> SHMKFTVEREHLLKPLQQVSGPLGGRPTLP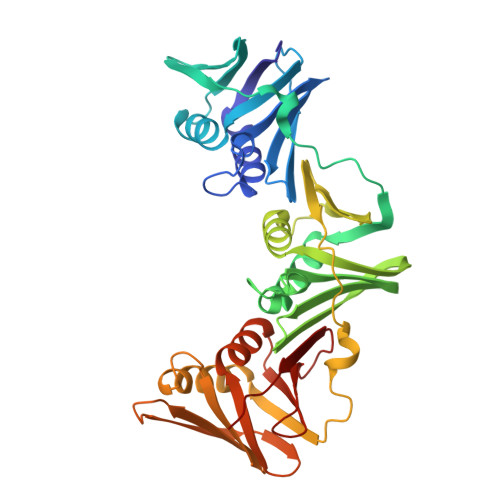ILGNLLLQVADGTLSLTGTDLEMEMVARVALVQPHEPGATTVPARKFFDICRGLPEGAEIAVQLEGERMLVRSGRSRFSLSTLPAADFPNLDDWQSEVEFTLPQATMKRLIEATQFSMAHQDVRYYLNGMLFETEGEELRTVATDGHRLAVCSMPIGQSLPSHSVIVPRKGVIELMRMLDGGDNPLRVQIGSNNIRAHVGDFIFTSKLVDGRFPDYRRVLPKNPDKHLEAGCDLLKQAFARAAILSNEKFRGVRLYVSENQLKITANNPEQEEAEEILDVTYSGAEMEIGFNVSYVLDVLNALKCENVRMMLTDSVSPVQIEDAASQSAAYVVMPMRL> AQSVPYGVSQIKAPALHSQGYTGSNVKVAVIDSGIDSSHPDLKVAGGASMVPSETNPFQDNNSHGTHVAGTVAALNNSIGVL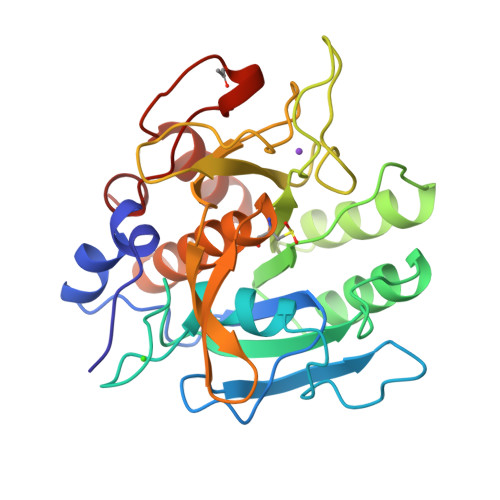GVAPSASLYAVKVLGADGSGQYSWIINGIEWAIANNMDVINMSLGGPSGSAALKAAVDKAVASGVVVVAAAGNEGTSGSSSTVGYPGKYPSVIAVGAVDSSNQRASFSSVGPELDVMAPGVSIQSTLPGNKYGAYSGTCMASPHVAGAAALILSKHPNWTNTQVRSSLENTTTKLGDSFYYGKGLINVQAAAQ>[2x]GSHMAPSRKFFVGGNWKMNGRKQSLGELIGTLNAAKVPADTE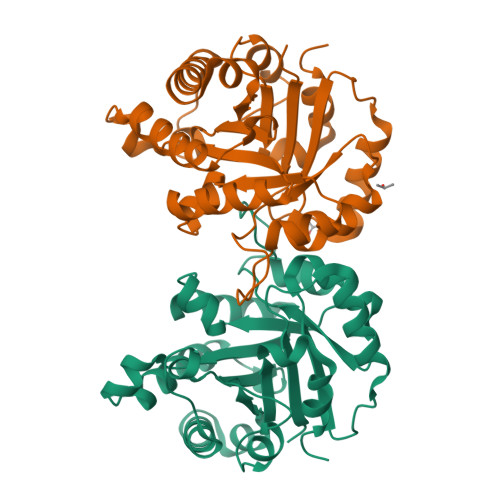VVCAPPTAYIDFARQKLDPKIAVAAQNCYKVTNGAFTGEISPGMIKDCGATWVVLGHSERRHVFGESDELIGQKVAHALAEGLGVIACIGEKLDEREAGITEKVVFEQTKVIADNVKDWSKVVLAYEPVWAIGTGKTATPQQAQEVHEKLRGWLKSNVSDAVAQSTRIIYGGSVTGATCKELASQPDVDGFLVGGASLKPEFVDIINAKQ>PEDELKRVEKLVKEAEMLLMLAKIKGSEKDLEKALRTAEEAAREAKKVLEQAEKEGDPEVALRAVELVVRVAELLLRIAKESGSEEALMTALLVAVVAATLAVRVLVLAAVQGDPEVALRAVELVVRVAELLLRIAKESGSEEALERALRVAEEAARLAKRVLELAQEQGDPVVAIAAVMLVKRVAELLERIARES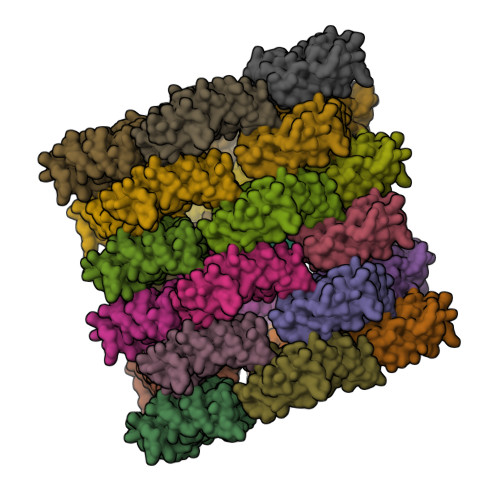GSEEAKERAERVREE[26x]>HESETTTSLVLERSLNRVHLLGRVGQDPVLRQ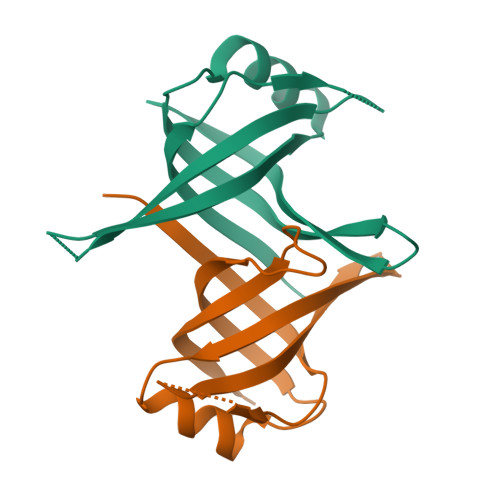VEGKNPVTIFSLATNEMWRSGDSEVYQLGDVSQKTTWHRISVFRPGLRDVAYQYVKKGSRIYLEGKIDYGEYMDKNNVRRQATTIIADNIIFLSDQTKEKE[2x]>[2x]MAHHHHHHMAEFSIIDQYFNRQSHPDVALGIGDDSALITPPPNQQLVICADTLVAGRHFPLETSPHAIGWKSVAVNLSDIAAMGAKPHSILLAISLPQVDHEWLEGFSQGIYDCCNQFGVALIGGDTTQGPHLTITVTAMGWIETGKAVLRSGAKVGDYVCVSGQIGDAAYGLQHLGHSLQQRLDYPTPRCKLGEELKG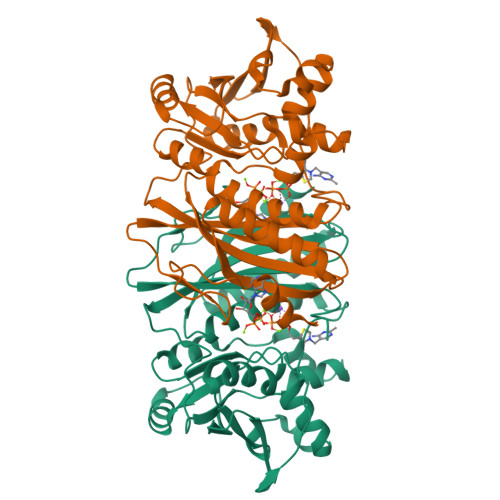LASSMIDVSDGLAQDLGHILKASKVGARLILEKLPVDPVLQQIEEQQRWQYALAGGDDYELCFTITPQNYEKLLQKQLDVKITMIGQIVEQTKLTFEHLGSDYPLQIHGYQHFA> MESLSEVSVQFSQLSMFPFFDMAHYLASVMSAREQAGALDIASHSPMASWFSAMLHCFGGGILSSILLAEPPVGILANTTNIMLASAIWYMVYYFPYDLFYNCFFFLPIRLIAAGMKEVTRTWKILSGITHAHSHYKDAWLVMITIGWARGAGGGLISNFE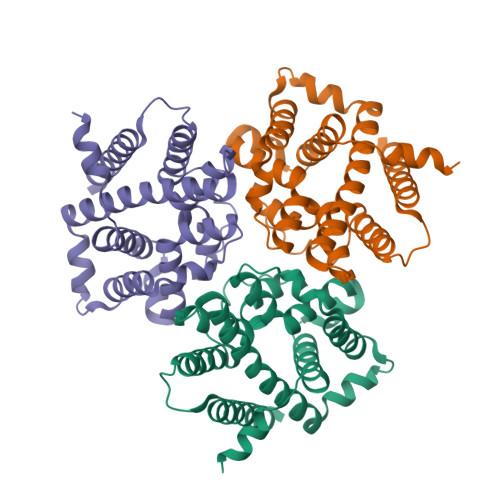QLVRGVWKPESNEFLKMSYPVKVTLIGAVLFTLQHGHYLPISRHNLMFIYTMFLVSIKVTMMLTHSAGSPFLPLETPLHRILFGLRQNQAEVRESPSSSGAKGKPSKKTLDKDSGEQSNKKDKAAAENLYFQGLEDYKDDDDKHHHHHHHHHH> TVMRELYLIDKNGYVVAQTLPLPKSESTAKQALEYLVQGGPVSEILPNGFRAVLPADTTVNVDIKKD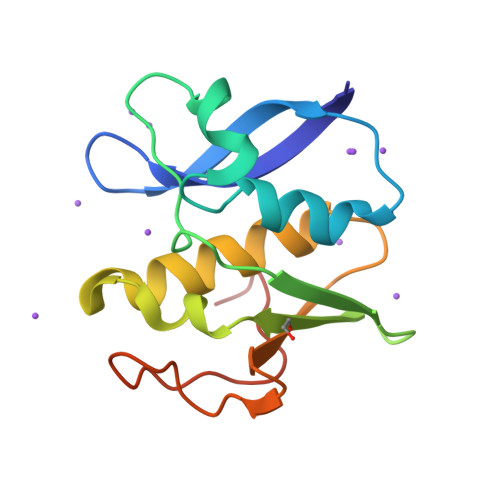GTAIADFSNEFKNYKKEDEQKIVQSVTWTLTQFSSIDKVKLRINGHELKEMPVGGTPISDDLSRKDGINLE>[2x]TSLKPTAIESCMVKFELSSSKWHMTSPKPHCVNTTSDGKLKILQSGTYLIYGQVIPVDKKYIKDNAPFVVQIYKKNDVLQTLMNDFQILPIGGVYELHAGDN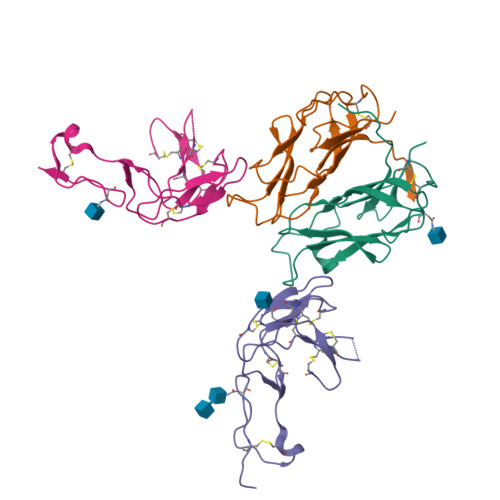IYLKFNSKDHIQKTNTYWGIILMPDLPFIS;>QPSVVEEPGCGPGKVQNGSGNNTRCCSLYAPGKEDCPKERCICVTPEYHCGDPQCKICKHYPCQPGQRVESQGDIVFGFRCVACAMGTFSAGRDGHCRLWTNCSQFGFLTMFPGNKTHNAVCIPEPLPTEQYGH[2x]> NLYFQSNAMKHCPITYEKISDQENYSQRGLHLLSPQLKNLSPLDLSADEQRQEAIARVGKMSVQGVQKKLSAKLKIKEGCFEIVDQYGQYILKPQSDIYPELPENEAITMTLAKTIGLEVPVHGLVYSKDNSLTYFIKRFDRIGHNKKLALEDFAQLSGEDRHTKYKSSMEKVIAVIEQFCTFPKIEFVKLFKLTLFNFLVGNEEMHLKNFSLITKDRKISISPAYDLLNSTIAQKNTKEELALPLKGKKNNLTKSDFLKYFAIEKLGLNQNVIDGIVQEFHQVIPKWQELIGFSFLSQEMQEKYLELLEQRCKRLNFFD

Here, we perform structural and biochemical characterization of the Legionella pneumophila effector Lpg2370, demonstrating that it is a Ser/Thr kinase. Together with two upstream genes, lpg2370 constitutes the tripartite HipBST TA. Notably, the toxin Lpg2370 (HipTLp) and the antitoxin Lpg2369 (HipSLp) correspond to the C-terminus and N-terminus of HipA from HipBA TA, respectively. Structural analysis reveals that HipSLp binding induces a loop-to-helix shift in the P-loop of HipTLp, leading to the blockage of ATP binding and inhibition of the kinase activity.

To elucidate how pHipTLp binds ATP, we determined the crystal structure of pHipTLp in complex with AMP–PNP at 1.36 Å resolution. The structure of pHipTLp–ATP reveals that AMP–PNP is bound to the P-loop like in other representative kinases. The backbone of pHipTLp in the complex is virtually identical to the apo structure (RMSD = 0.35 Å), with the exception of P-loop that bends towards helix α2 to accommodate the AMP–PNP. In pHipTLp, the γ-phosphate of AMP–PNP is stabilized by V58, H199, and D219, the β-phosphate forms hydrogen bonds with Q59, K61, and K85, whereas the α-phosphate interacts with K85 and N202. The adenosine moiety interacts with the main chain of K130 and forms π-stacking interactions with the side chain of F132. ATP (AMP–PNP)-interacting residues appear to be conserved among the bacterial HipT toxins, implying a shared mechanism for ATP binding. Thermal shift assays performed with the purified wild-type HipTLp revealed a 2.5 °C-increase in the melting temperature (Tm) in the presence of non-hydrolysable ATP analogue adenylyl-imidodiphosphate (AMP–PNP), suggesting that pHipTLp indeed binds ATP. Taken together, these results suggest that unlike in E. coli HipA, HipT retains the ATP-binding ability independent of the autophosphorylation on the conserved S54 in the P-loop and that HipT uses a universal mode for ATP recognition.Histopine | C9 H13 N3 O4 | 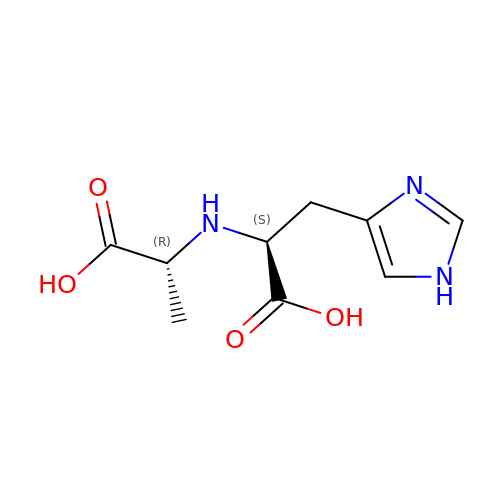KEMGAOPOGGLPBQ-VDTYLAMSSA-N>MANSERTFIAIKPDGVQRGLIGEII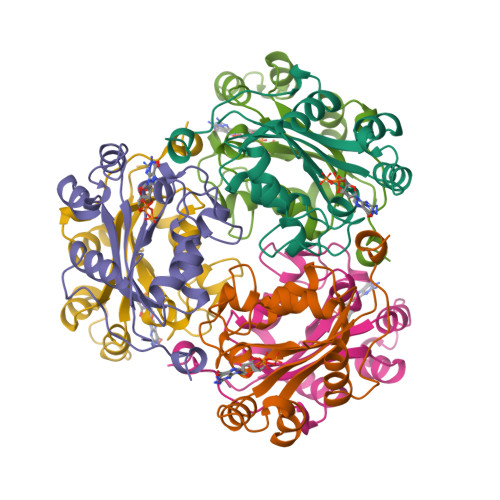KRFEQKGFRLVAMKFMRASEDLLKEHYIDLKDRPFFAGLVKYMHSGPVVAMVWEGLNVVKTGRVMLGETNPADSKPGTIRGDFCIQVGRNIIHGSDSVESAEKEIALWFHPEELVNYKSCAQNWIYE[6x]>MSSLRPAQSSSSSSRTRQSSQARILAQTTLDAELNAEYEESGDSFDYSKLVEAQRSTPPEQQGRSGKVIAYLQHIQRGKLIQPFGCLLALDEKSFRVIAFSENAPEMLTTVSHAVPNVDDPPKLGIGTNVRSLFTDPGATALQKALGFADVSLLNPILVQCKTSGKPFYAIVHRATGCLVVDFEPVKPTEFPATAAGALQSYKLAAKAISKIQSLPGGSMQALCNTVVKEVFDLTGYDRVMAYKFHEDEHGEVFAEITKPGIEPYLGLHYPATDIPQAARFLFMKNKVRMICDCRARSVKIIEDEALS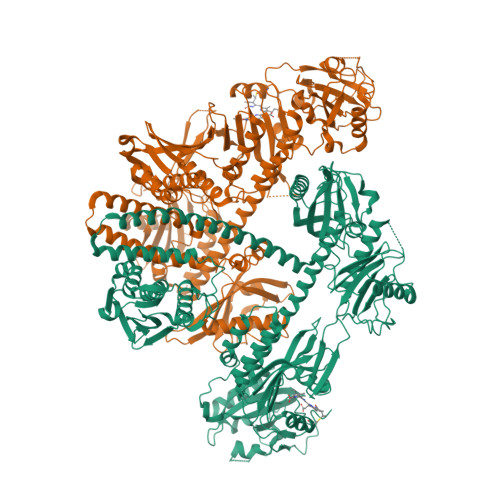IDISLCGSTLRAPHSCHLQYMENMNSIASLVMAVVVNENEDDDEPESEQPPQQQKRKKLWGLIVCHHESPRYVPFPLRYACEFLAQVFAVHVNKEFELEKQIREKSILRMQTMLSDMLFKESSPLSIVSGSPNIMDLVKCDGAALLYGDKVWRLQTAPTESQIRDIAFWLSEVHGDSTGLSTDSLQDAGYPGAASLGDMICGMAVAKITSKDILFWFRSHTAAEIKWGGAKHDPSDEDDSRRMHPRLSFKAFLEVVKMKSLPWSDYEMDAIHSLQLILRGTLNDALKPAQSSGLDNQIGDLKLDGLAELQAVTSEMVRLMETATVPILAVDGNGLVNGWNQKVADLSGLRVDEAIGRHILTLVEDSSVPIVQRMLYLALQGREEKEVRFELKTHGSKRDDGPVILVVNACASRDMHDHVVGVCFVAQDMTVHKLVMDKFTRVEGDYRAIIHNPNPLIPPIFGADQFGWCSEWNAAMTKLTGWHRDEVIDRMLLGEVFDSSNASCLLKSKDAFVRLCIIINSALAGEEAEKAPIGFFDRDGKYIECLLSVNRKVNADGVVTGVFCFIHVPSDDLQHALHVQQASEQTALRRLKAFSYMRHAIDKPLSGMLYSRETLKGTDLDEEQMRQVRVADNCHRQLNKILADLDQDNITDKSSCLDLDMAEFVLQDVVVSAVSQVLIGCQGKGIRVACNLPERSMKQKVYGDGIRLQQILSDFLFVSVKFSPAGGSVDISSKLTKNSIGENLHLIDFELRIKHQGAGVPAEILSQMYGEDNREQSEEGLSLLVSRNLLRLMNGDIRHLREAGMSTFILTAELAAA[2x]>MLKKNDIVEVEIVDLTHEGAGVAKVDGLVFFVENALPSEKILMRVLKVNKKIGFGKVEKYLVQSPHRNQDLDLAYLRSGIADLGHLSYPEQLKFKTKQVKDSLYKIAGIADVEVAETLGMEHPVKYRNKAQVPVRRVNGVLETGFFRKNSHNLMPLEDFFIQDPVIDQVVVALRDLLRRFDLKPYDEKEQSGLIRNLVVRRGHYSGQIMVVLVTTRPKVFRVDQLIEQVIKQFPEIVSVMQNINDQNTNAIFGKEWRTLYGQDYITDQMLGNDFQIAGPAFYQVNTEMAEKLYQTAIDFAELKKDDVIIDAYSGIGTIGLSVAKHV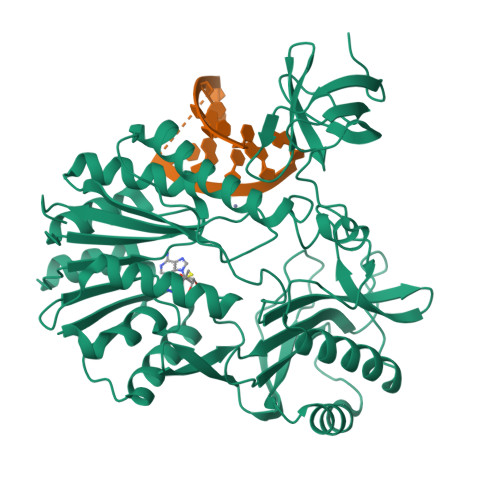KEVYGVELIPEAVENSQKNASLNKITNAHYVCDTAENAMKKWLKEGIQPTVILVDPPRKGLTESFIKASAQTGADRIAYISCNVATMARDIKLYQELGYELKKVQPVDLFPQTHHVQTVALLSKLDVD[4x]> MRGSTRDQNGTWEMESNENFEGYMKALDIDFATRKIAVR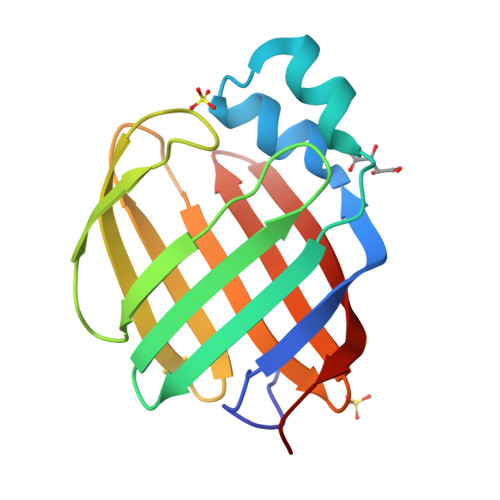LTQTKVIDQDGDNFKTKTTSTFRNYDVDFTVGVEFDEYTKSLDNRHVKALVTWEGDVLVCVQKGEKENRGWKQWIEGDKLYLELTCGDQVCRQVFKKKLVPR>[2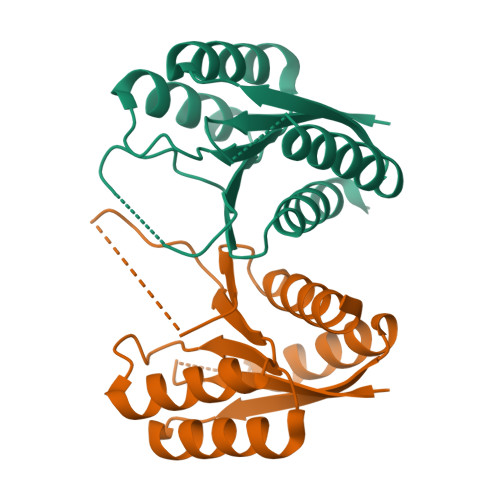x]SNAMTKVIVVNGPNLGRLGVRQPDVYGRQDLDTLRKLCAEWGKDLGLEVEVRQTDDEAEMVRWMHQAADEKTPVVMNPAAFTHYSYALADAAHMVIDENLPLMEVHISNPSARDEFRKRSVISPVATGTITGMGFYGYKLALDAVAHLLSE> MGDSILSQAEIDALLNGDSDTKDEPTPGIASDSDIRPYDPNTQRRVVRERLQALEIINERFARQFRMGLFNLLRRSPDITVGAIRIQPYHEFARNLPVPTNLNLIHLKPLRGTGLVVFSPSLVFIAVDNLFGGDGRFPTKVEGREFTHTEQRVINRMLKLALEGYSDAWKAINPLEVEYVRSEMQVKFTNITTSPNDIVVNTPFHVEIGNLTGEFNICL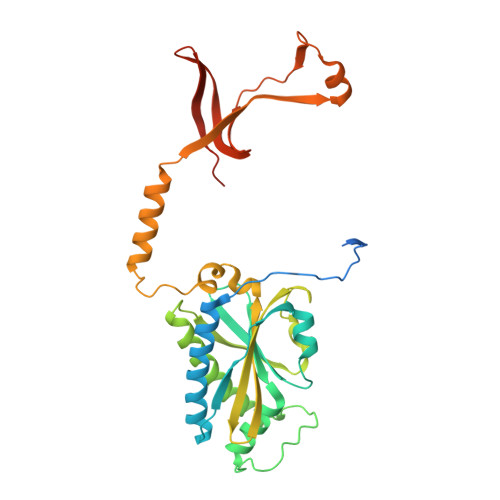PFSMIEPLRELLVNPPLENSRHEDQNWRDNLVRQVQHSELELVANFADIPLRLSQILKLKPGDVLPIEKPDRIIAHVDGVPVLTSQYGTVNGQYALRVEHLINPILNSLNEEQPK>MSKQQYRLGIDAGGTFTDFILADHQGNVQLFKAPSTPHDGTLAIRNGLAQIADALGRTPAEIIADCDLCINGTTVALNALIEKTGVKVGLLCTDGHEDSLEIRLGHKEDGHRYDATYPPAHMLVPRHLRRPIGGRIISDGSEFSPLDEAAIHAAIDYFREQQVQAVAISFVWSVRNPSHEQRAMAMVRAALPDVFVCSGHEVFPQIREYTRTSTTVVNAYLSPVMGRYIERIDALFEELGAQQPTRYFQSNGGLAPGVVMRERAVNAINSGPASAPQAGLCVAQPFGIDNVITVDMGGTSFDITLSKGGRTNFSKDSDFLRYRIGVPMIQVETLGAGGGSIAHLDDFGMLQVGPRSAGANPGPVCYGKGGVEPTVTDANLALGYLADGALLGGSIRLNRQAAIDAIRSKIAEPLGISVERAAVGIITLVNLSMVSGIRRVSIERGYDPRDFALIGAGGAAGMHVMRLAEEIGSKVVLIPKVASGLCAFGQILSDIRYDQLTTLPMRLDDEFVDLEQLNQALQQLRERGMTNLRDDGFGGDNRIECQYSLEIRYLGQIHECSVELSCDRLDRSSLAALRESFHQRHKALFSYSEPNSPVELVNLECSVIARLQRPPMPELATPLKATAAIPAGHRPMLFNAQDDWQDTPVYNGDRIEVGQIIQGPCVIEEATTNILVPPGWRVSLDPSATYELTPGH[2x];>MNTVDPITLAVVRGALETAQREMTLTLEKTSRSSVFNLAHDYSNALFDHLPEMILQGQDIPIHLGSLIPAMKCVAGFFGDEIAEGDVIYHNDPAYMGSHILDCCMYKPVFYKGELVFWTVCKGHLTDIGGPVPAGYNPDAKEIYAEGLRIPPVKLWAQGQRREDVINLLLTNMRARAYQEGDLNAQYGACSVGERHLIELLDRYGVDQVRACITELKDMADRHMRALLRDVPDGFYSGTAILEDSGHGLGELSITAQVEIRGDEAHVLIESPPQVPYFINSYAGNSISGVYLGLMMFAQVPPPYNEGLYRCVSVDLGPSGTLCNAQEPAPHVNCTTTPMETLADAVRLALEQAAPERVTASWGHASGINIAGHDPRNNNDEYVTMVLASVISGAGANKAMDGWPACGPLCCFGALMSGDIELLEYSYPVLIHRYSLMTDSGGA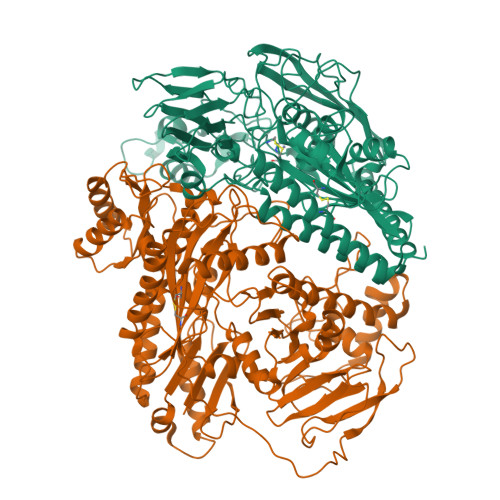GEFRGGSGTRLELEPLKHAMTVVGFGEGRQLPTAGAAGAKNVLLEPKLGRLIHRHVDGEEDHYIQNTLLTAQPGERVINVNPGGGGYGDPLRRPLATVLADVRNGLVSIDGARLEYGVVIDGNGQLDEAATHAHRAAH[2x]>[2x]GMNPAAEAEFNILLATDSYKVTHYKQYPPNTSKVYSYFECRE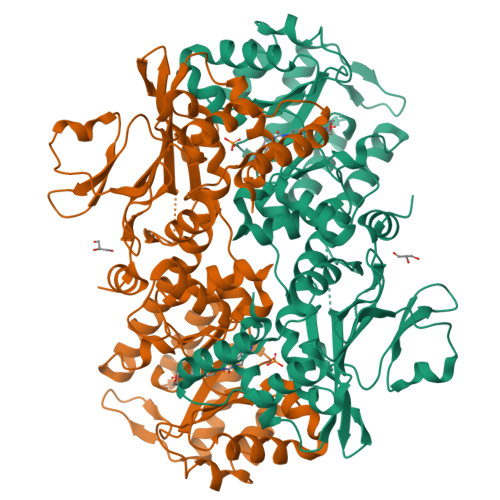KKTENSKLRKVKYEETVFYGLQYILNKYLKGKVVTKEKIQEAKDVYKEHFQDDVFNEKGWNYILEKYDGHLPIEIKAVPEGFVIPRGNVLFTVENTDPECYWLTNWIETILVQSWYPITVATNSREQKKILAKYLLETSGNLDGLEYKLHDFGYRGVSSQETAGIGASAHLVNFKGTDTVAGLALIKKYYGTKDPVPGYSVPAAEHSTITAWGKDHEKDAFEHIVTQFSSVPVSVVSDSYDIYNACEKIWGEDLRHLIVSRSTQAPLIIRPDSGNPLDTVLKVLEILGKKFPVTENSKGYKLLPPYLRVIQGDGVDINTLQEIVEGMKQKMWSIENIAFGSGGGLLQKLTRDLLNCSFKCSYVVTNGLGINVFKDPVADPNKRSKKGRLSLHRTPAGNFVTLEEGKGDLEEYGQDLLHTVFKNGKVTKSYSFDEIRKNAQLNIELEAAHH> XNLAALRSELQALRREGFSPERLAALESRLQALERRLA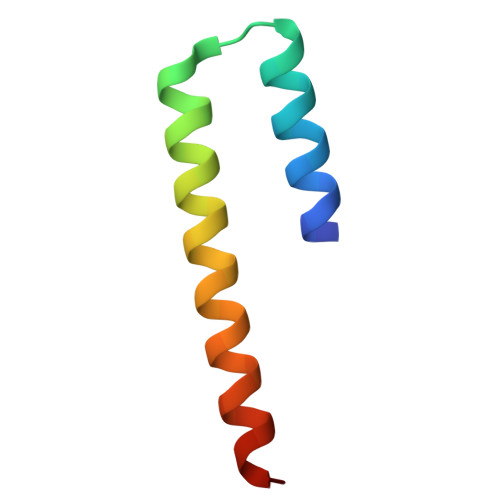ALRSRLQALRGX>[3x]AMKIGVIGAGTMGQGIAKAFAQVEGNTVALCDIKQEWAENGLAKIKKGYEKLVAKGKIPQEKADAIVAAITPGLKENLCADCDLIVEAAFEDMKVKQTTFGELDKICKPECIFASNTASLSITEIGKGLSRPLVGMHFFNPADRMKLIEVIAGCNTPAETVEKIKEISVAIGKNPVQVNEAAGFVVNRILIPMINEAAFIKMEGVSDIAGIDTAMKL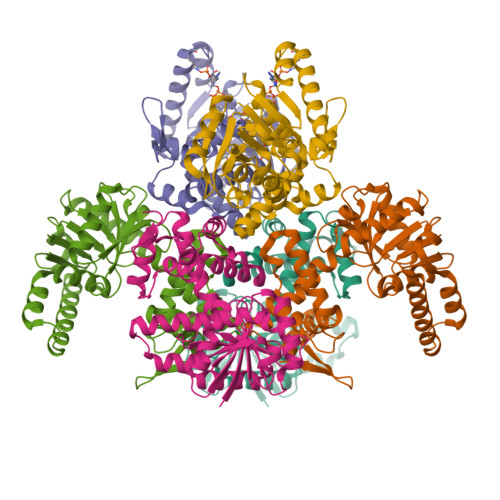GANHPMGPLELGDFIGLDICLAIMDVLYHETGDSKYRACPLIRKMVRGGNLGCKTGKGFYVYNADRTKTPVDN> AP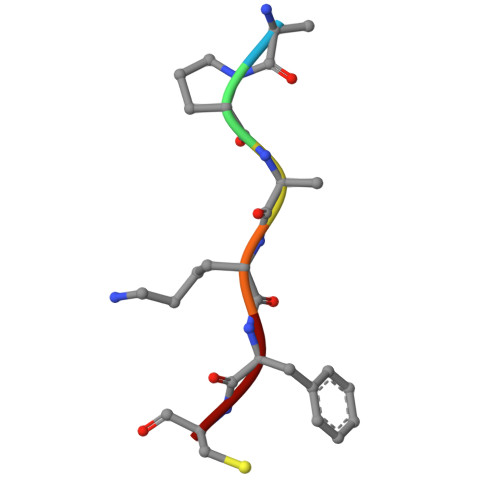AKFC> MENNDLYQAAIGWYRAFEDCPPELHLCCPKVDDDDYATYDEPDVVDDSGVPVEEKKRRISAYEERFQNVYNLSILLGLGKEVAGPWLDEWTRAVDSLLKKCDTCVRNWHRNRDPYLKALHLSPEQVTYLQSKLDEFDRQRITEGLQRAKAILEQYGPMSTVKLVDHDMSAVLALYEALCSLPYLARPEHQPLFDFVFENTQRKKPLRMQGGIIPSMTLFLFDESPVRRRFAETAWENRQPGSITAQEWDWAISGRLADQIVSLSFNRLQTLPPGQKILRFWSGFLFILHALSEKQIINSLRAMEVSPSIYFLALEHLGTNSDEALAMVLRALQELMEKSSKAFWQALEQVPPNQLVEEIFKSAAFRPLLNKSLRPELLVTEGDSQVPALAAWMRALVRSLPSTSWSDLCETSLRHLFETFRSDQAVDQSGRATCTLAGLVTLQQCLDGFLQQDSIDTGTGLIMVNQLLNRVVNYSEIIIRAASLKPGDIYNVGISKAAMAIIHSALALDAKATEVEWAALIAEKPVQDAVNRDSGALWETFLEMLWAGQLGHFELAKAMLMATLRLRSIEQFIPKRKEQLKRELDKFNKRYQQQTTAIGKMLNRLTDFEPEVLDKLCSDPRGQTIHPIVSSLIHGEDAIREAGFQLLKAITSESQPSDAVGRMLEVYFTPFLNAFSQAVDKLTATKDANSPWSHMIPILKCSDFVLTGLCDPSSGQLRRKVLTTEEHAAVKRWWECVWQAVDHSFRMMRIWHIKIDKKVMEDFCRDVMELGNKLLAQDGVMASSLAQESGEDAISKAMREVLDPPRKCSYSLADMLQLRDKYLVMGIIETIKKLLSRLQENEMNLPQRTRGHLDSMLKKTKQRDGRMDYLTKTNLTDVQRIELLKALGEDAVIEEQFMGTKPGDREAKEKERALKQSKLDFSKAGISYSGDINEHLAQITPNFEKYHKSSLLETLKKEEPAKPKAPAKLSQQAILANQQQIKEARARERAEKARRDAEAIAKAKALRAGKTIPGEGSGLQSIAGVRGKDHAPVVKDEIMVGSSSEDEGDDDDDDDVINRAKTKSKKIWDEAERRRLELEAEKLRGPVKKMKILRSAKDMRARLIPPMDVLHQAILEWDIFHEGNDPPNGYRCGNVSDTYPDPYSYKQTFFPLLINEAWRSFVTAKDETTSKPFGIKVLSRMTVDKFMEVTAAVPAQISKDRGLTEGDIVIISKGEDPLNQPQELHCLSRIWKTTYKKDTVEVVYRLNAKGNQILPALTPGSEFQVVKITNMTTIEREYAALESLQYYDLMDEILKAQPSPMLTFGDEAIKAVMDNYQLNPGQARAILNAKENDGFTLIQGPPGTGKTKTIVAMVGCLLTGVLKSSNTGAVQISRPGAGPTNGTAPSKKLLVCAPSNAAVDELVLRLKAGVKTMNG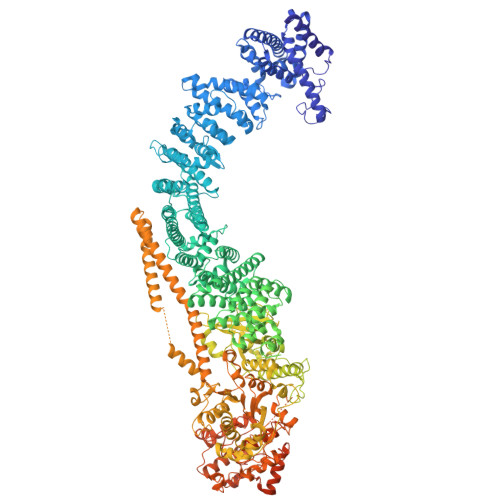TFHKIEVLRLGRSDVINAAVKDVTLDELVKARMDAELSKNSSPSERDQLHKEAGEIKAKLAEIRPQLDAARLSDDRASAMKLQREFDELKRRQAHIGAKIDADKASGNTYARETEIKRRQIQQEILDKAQVLCATLSGSGHEMFKNLNVEFETVIIDEAAQCVELSALIPLKYGCNKCILVGDPKQLPPTVLSQSAAKYGYDQSLFVRMQKNHPKDVHLLDMQYRMHPEISRFPSKEFYEGLLQDGADMARLRLQPWHQSVLLGPYRFFDVKGSQERGPKNQSLVNEEEVKVAMQLYMRFRSDYRDIDLTGKIGIITPYKAQLQRLRQKFVERYGESITEQIEFNTTDAFQGRECEIIIFSCVRASPTGGIGFMTDIRRMNVGLTRARSSLWILGDSRALVQGEFWAKLIEDAKQRDRYTNGNIMALLSQPGPRVSLESLAKQYSVPVAPVARSKEDVEMHDTPRTSESIPPAMPYRGSGIGGLNERGEATTPTTRGGELPIIQSTDGSAGKKRPRDANEENRPAFDPAKASSAFWFTQTTGIGIGIDRSFCDGSFGAGSSNPSASSATATPSSSGTF> SSRTRRE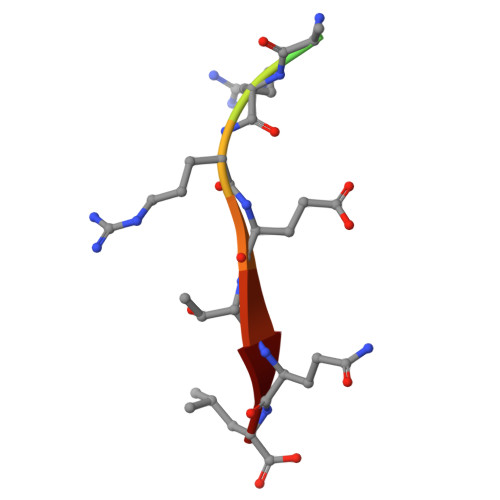TQL> MSKILVIAEHRRNDLRPV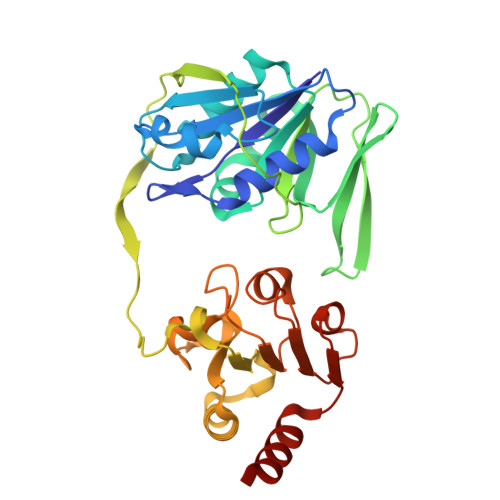SLELIGAANGLKKSGEDKVVVAVIGSQADAFVPALSVNGVDELVVVKGSSIDFDPDVFEASVSALIAAHNPSVVLLPHSVDSLGYASSLASKTGYGFATDVYIVEYQGDELVATRGGYNQKVNVEVDFPGKSTVVLTIRPSVFKPLEGAGSPVVSNVDAPSVQSRSQNKDYVEVGGGNDIDITTVDFIMSIGRGIGEETNVEQFRELADEAGATLCCSKPIADAGWLPKSRQVGQSGKVVGSCKLYVAMGISGSIQHMAGMKHVPTIIAVNTDPGASIFTIAKYGIVADIFDIEEELKAQLAA>AATERLSLGS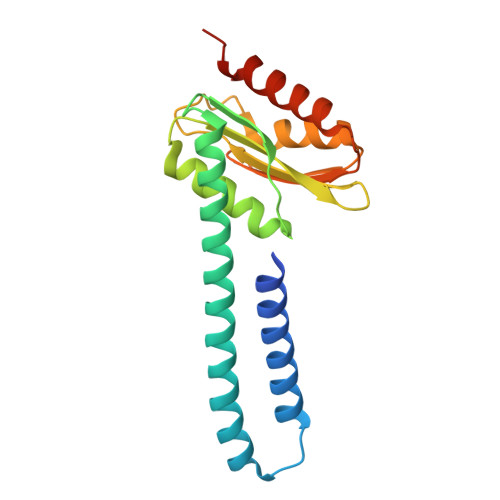RDVAEALRLSKDIGRLIEAVETAVMPQWQRRELLATVKMLQRRANTAIRKLQMGQAAKKTQELLERHSKGPLIVDTVSAESLSVLVKVVRQLCEQAPSTSVLLLSPQPMGKVLCACQVAQGAMPTFTAEAWALAVCSHMGGKAWGSRVVAQGTGSTTDLEAALSIAQTYALSQLLEHHHHHH[4x]>[4x]MDLTVEPNLHSLITSTTHKWIFVGGKGGVGKTTSSCSIAIQMALSQPNKQFLLISTDPAHNLSDAFGEKFGKDARKVTGMNNLSCMEIDPSAALKDMNDMAVSRANNNGSDGQGDDLGSLLQGGALADLTGSIPGIDEALSFMEVMKHIKRQEQGEGETFDTVIFDTAPTGHTLRFLQLPNTLSKLLEKFGEITNKLGPMLNSFMGAGNVDISGKLNELKANVETIRQQFTDPDLTTFVCVCISEF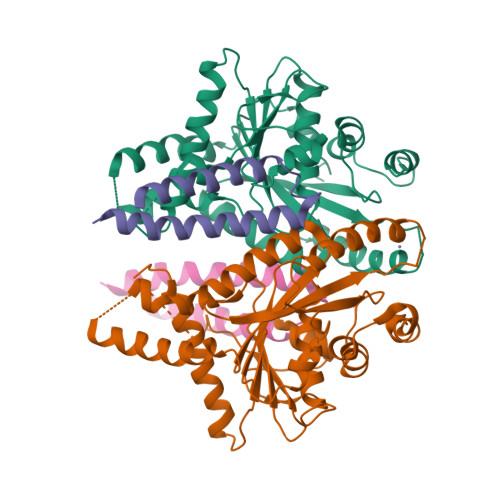LSLYETERLIQELISYDMDVNSIIVNQLLFAENDQEHNCKRCQARWKMQKKYLDQIDELYEDFHVVKMPLCAGEIRGLNNLTKFSQFLNKEYNPITDGKVIYELEDKELEHHHHHH;>[4x]MNELSKKYLAKVKERHELKEFNNSISAQDNYAKWTKNNRKLDSLDKEINNLKDEIQSENHHHHHH>AQDMVSPPP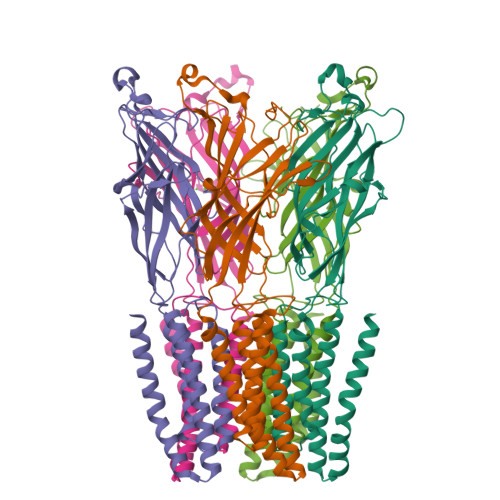PIADEPLTVNTGIYLIECYSLDDKAETFKVNAFLSLSWKDRRLAFDPVRSGVRVKTYEPEAIWIPEIRFVNVENARDADVVDISVSPDGTVQYLERFSARVLSPLDFRRYPFDSQTLHIYLIVRSVDTRNIVLAVDLEKVGKNDDVFLTGWDIESFTAVVKPANFALEDRLESKLDYQLRISRLYFSYIPNIILPMLFILFISWTAFWSTSYEANVTLVVSTLIAHIAFNILVETNLPKTPYMTYTGAIIFMIYLFYFVAVIEVTVQHYLKVESQPARAASITRASRIAFPVVFLLANIILAFLFFGF[5x]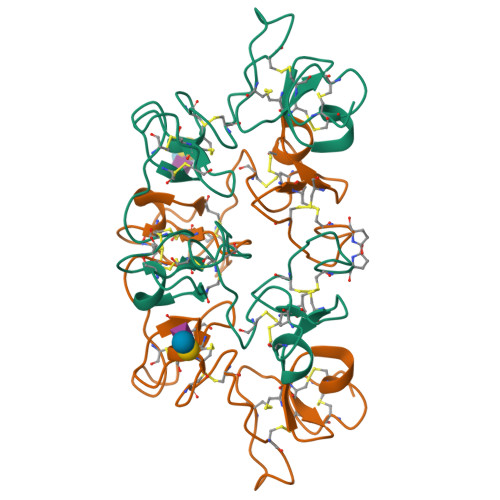>QRCGEQGSNMECPNNLCCSQYGYCGMGGDYCGKGCQNGACWTSKRCGSQAGGATCPNNHCCSQYGHCGFGAEYCGAGCQGGPCRADIKCGSQSGGKLCPNNLCCSQWGFCGLGSEFCGGGCQSGACSTDKPCGKDAGGRVCTNNYCCSKWGSCGIGPGYCGAGCQSGGCDA[2x]>[2x]PLGSEFKGLRRRRKCEKAGCTATCPVCFASASERCAKNGYTSRWYHLSCGEHFCNECFDHYYRSHKDGYDKYTTWKKIWTSNGKTEPSPKAFMADQQLPYWVQCTKPECRKWRQLTKEIQLTPQIAKTYRCGMKPNTAIKPETSDHCSLPEDLRVLEVSNHWWYSMLILPPLLKDSVAAPLLSAYYPDCVGMSPSCTSTNRAAATGNASPGKLEHSKAALSVHVPGMNRYFQPFYQPNECGKALCVRPDVMELDELYEFPEYSRDPTMYLALRNLILALWYTNCKEALTPQKCIPHIIVRGLVRIRCVQEVERILYFMTRKGLINTGVLSVGADQYLLPKDYHNKSVIIIGAGPAGLAAARQLHNFGIKVTVLEAKDRIGGRVWDDKSFKGVTVGRGAQIVN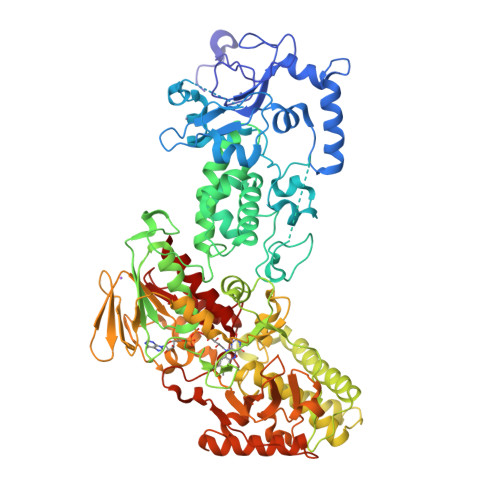GCINNPVALMCEQLGISMHKFGERCDLIQEGGRITDPTIDKRMDFHFNALLDVVSEWRKDKTQLQDVPLGEKIEEIYKAFIKESGIQFSELEGQVLQFHLSNLEYACGSNLHQVSARSWDHNEFFAQFAGDHTLLTPGYSVIIEKLAEGLDIQLKSPVQCIDYSGDEVQVTTTDGTGYSAQKVLVTVPLALLQKGAIQFNPPLSEKKMKAINSLGAGIIEKIALQFPYRFWDSKVQGADFFGHVPPSASKRGLFAVFYDMDPQKKHSVLMSVIAGEAVASVRTLDDKQVLQQCMATLRELFKEQEVPDPTKYFVTRWSTDPWIQMAYSFVKTGGSGEAYDIIAEDIQGTVFFAGEATNRHFPQTVTGAYLSGVREASKIAAF At the core of this natural phenomenon lies a fundamental process of energy transduction by luciferase enzymes that convert the chemical energy stored within the ground-state substrate (luciferin) to an excited, emissive state of the product (oxyluciferin) by a spin-forbidden process. Although beetle luciferase systems share identical substrates and chemical reaction sequence, they emit a range of different colors from yellow green (λmax ≈ 560 nm), which is typical for common firefly species, such as the North American firefly Photinus pyralis (GPp) and the Japanese firefly Luciola cruciata (GLc), to orange and even red (λmax = 590–623 nm) from certain click beetles and railroad worms. Here, we describe the first crystal structures of two rare WT luciferases from Brazilian beetles that emit light with exceptional colors; a luciferase from the head lanterns of the glow-worm P. hirtus (Coleoptera: Phengodidae), the only known luciferase that naturally emits red light (λmax = 623 nm; REPh), and a green-emitting luciferase from the firefly A. vivianii (Coleoptera: Lampyridae) that displays a blue-shifted emission relative to common firefly luciferases (λmax = 538 nm at pH 8; GBAv). Biochemical and structural analyses of the two luciferases, combined with computational modeling, provide the best insight yet into the relationship between the structure and color of light emitted by beetle luciferases.

The crystal structure of WT REPh was determined at low resolution by molecular replacement from two different crystal forms in the space groups P1 and P3121 at resolution of 3.05 Å and 3.60 Å, respectively. Unlike previously reported luciferases that are exclusively monomeric, in the P3121 crystal form, REPh exists as tetramer, although in the P1 crystal form it is an octamer in the asymmetric unit. The estimated molecular weight (MW) of the wild-type (WT) REPh from the SEC analysis was ≈ 240 kDa, which corresponds to the tetramer found in the P3121 crystal. Only one out of the four C-terminal domains was observed in the density maps of the P3121 crystal form and none of the eight C-terminal domains of the REPh octamer could be resolved in the P1 crystal form. Only molecule B of the P3121 crystal form has enough quality to trace the C-terminal domain that was not traceable in any of the molecules in the P1 crystal form. The C-terminal domain showed higher average B factors (69.4 Å2, with several regions with values above 100) relative to the N-terminal domain within the same crystal form (60.3 Å2). The aperture of the active site with an angle of ∼125° between axes crossing the center mass of each domain (P3121 crystal form) shows that REPh is the most open conformation among the known luciferase structures, which corresponds to the high mobility of its C-terminal domain. This feature indicates that the flexibility of the C-terminal domain may play a role in tuning the color of light emitted.

>MEEENIVNGDRPRDLVFPGTAGLQLYQSLYKYSYITDGIIDAHTNEVISYAQIFETSCRLAVSLEKYGLDHNNVVAICSENNIHFFGPLIAALYQGIPMATSNDMYTEREMIGHLNISKPCLMFCSKKSLPFILKVQKHLDFLKKVIVIDSMYDINGVECVFSFVSRYTDHAFDPVKFNPKEFDPLERTALIMTSSGTTGLPKGVVISHRSITIRFVHSSDPIYGTRIAPDTSILAIAPFHHAFGLFTALAYFPVGLKIVMVKKFEGEFFLKTIQNYKIASIVVPPPIMVYLAKSPLVDEYNLSSLTEIACGGSPLGRDIADKVAKRLKVHGILQGYGLTETCSALILSPNDRELKKGAIGTPMPYVQVKVIDINTGKALGPREKGEICFKSQMLMKGYHNNPQATRDALDKDGWLHTGDLGYYDEDRFIYVVDRLKELIKYKGYQVAPAELENLLLQHPNISDAGVIGIPDEFAGQLPSACVVLEPGKTMTEKEVQDYIAELVTTTKHLRGGVVFIDSIPKGPTGKLMRNELRAIFAREQAKSKL[4x]>[2x]SNAMNRRVINPETMYPSVPFGFSHAVEQLSGRTLHIAGQ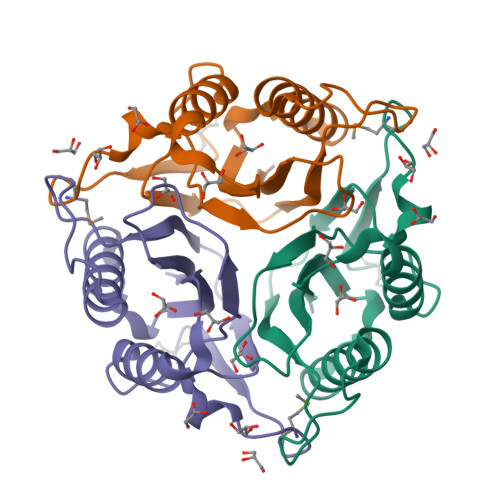VAWNANGELVGGQDLLAQTQQVLANLKEVLRYAGATPADVVRLRTYVVNHSPANLAAICAQIGAFYEGADPAANSFIGVQALALPELLIEIEATACLG Bromodomains (BRDs) are protein interaction modules that specifically recognize ε-N-lysine acetylation motifs, a key event in the reading process of epigenetic marks. The 61 BRDs in the human genome cluster into eight families based on structure/sequence similarity. Despite large sequence variations, all BRD modules share a conserved fold that comprises a left-handed bundle of four α helices (αZ, αA, αB, αC), linked by loop regions of variable length (ZA and BC loops), which line the Kac binding site and determine binding specificity. The four helices form a deep cavity that is extended by the two loop regions (ZA and BC loops), creating a largely hydrophobic Kac binding pocket.

BRDs are evolutionarily conserved and present in diverse nuclear proteins comprising HATs (GCN5, PCAF), ATP-dependent chromatin-remodeling complexes (BAZ1B), helicases (SMARCA), methyltransferases (MLL, ASH1L), transcriptional coactivators (TRIM/TIF1, TAFs) transcriptional mediators (TAF1), nuclear-scaffolding proteins (PB1), and the BET family (Muller et al., 2011). The most notable structural difference within the BRD core fold is a hairpin insertion located between helix αZ and the ZA loop that is present in all family VIII members. The proximity to the Kac binding site suggests that this insert may play a role in recruitment of acetylated binding partners. The nuclear body protein SP140 as well as the related protein LOC93349 and PCAF showed nonspecific binding to most peptides. In contrast, the second, fourth, fifth, and sixth BRD of PB1, MLL, and TRIM28 interacted with only a few histone Kac peptides.

>MGDSMISSATSDTGSAKRKSKKNIRKQRMKILFNVVLEAREPGSGRRLCDLFMVKPSKKDYPDYYKIILEPMDLKIIEHNIRNDKYAGEEGMIEDMKLMFRNARHYNEEGSQVYNDAHILEKLLKEKRKELGPLPDDDDMASPAENLYFQ[2x]>HHHHHHSSGLVPRGSHMMSTQFRMDSVPGSLVVVGGTYEPWLPVLEKVGWRCTQVADLRKPDALFVETGPCIGIVDLSHDEFSLNGIANLVSSHKQVRWLAFIREAQLSSDTICQFIVNFCIDFFTAPIPDAQLLSTIGHQLGMLKLEKKVWPHFGSAGNMGLIGESMPMKRLRDQIKRIGPTDVSILIYGESGTGKETVAKAIHKTSSRAQKPFISVNCRAMSEKRLESELFGLGETEEGQQPFLLQADGGTLLLNDILTLPKSQQLNLLRFLQEGTVETRQGVRAVDVRILAANSSDIEKALIDGDFNEELYHYINVLRINVPSLKERASDIVLLAKHFLQEYSKEYNAQARSFSDDAVRGLTRYHWPGNVRELMNQIKRVVLMSDTVVLDESQLDL[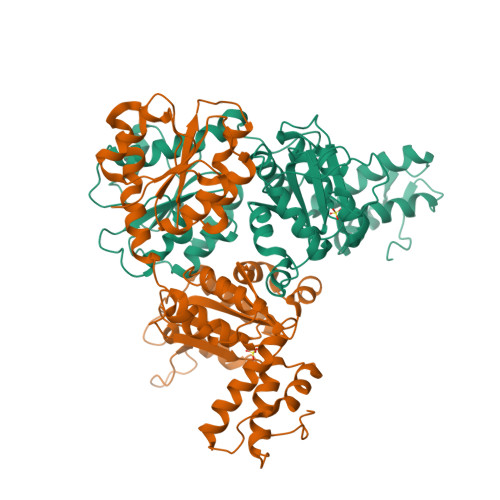2x]> DYVLYKDATKPVEDRVADLLGRMTLAEKIGQMTQIERLVATPDVLRDNFIGSLLSGGGSVPRKGATAKEWQDMVDGFQKACMSTRLGIPMIYGIDAVHGQNNVYGATIFPHNVGLGATRDPYLVKRI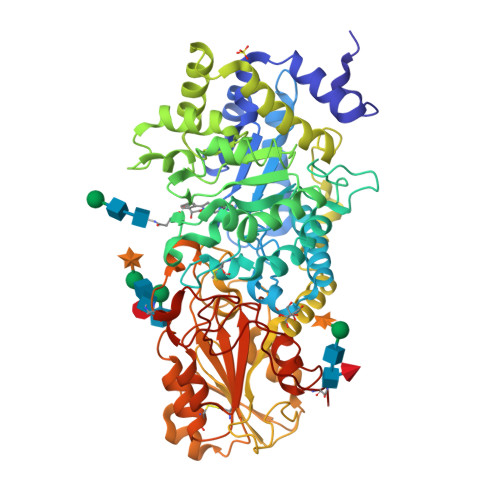GEATALEVRATGIQYAFAPCIAVCRDPRWGRCYESYSEDRRIVQSMTELIPGLQGDVPKDFTSGMPFVAGKNKVAACAKHFVGDGGTVDGINENNTIINREGLMNIHMPAYKNAMDKGVSTVMISYSSWNGVKMHANQDLVTGYLKDTLKFKGFVISDWEGIDRITTPAGSDYSYSVKASILAGLDMIMVPNKYQQFISILTGHVNGGVIPMSRIDDAVTRILRVKFTMGLFENPYADPAMAEQLGKQEHRDLAREAARKSLVLLKNGKTSTDAPLLPLPKKAPKILVAGSHADNLGYQCGGWTIEWQGDTGRTTVGTTILEAVKAAVDPSTVVVFAENPDAEFVKSGGFSYAIVAVGEHPYTETKGDNLNLTIPEPGLSTVQAVCGGVRCATVLISGRPVVVQPLLAASDALVAAWLPGSEGQGVTDALFGDFGFTGRLPRTWFKSVDQLPMNVGDAHYDPLFRLGYGLTTNAT> SHMNSEILNNIILNLRYRDNNLIDLSGYGANVEVYDGVELNDKNQFKLTSSTNSEIRVTQNQNIIFNSMFLDFSVSFWIRIPKYKNDGIQNYIHNEYTIINCIKNNSGWKISIRGNRIIWTLTDINGKTKSVFFEYSIREDISD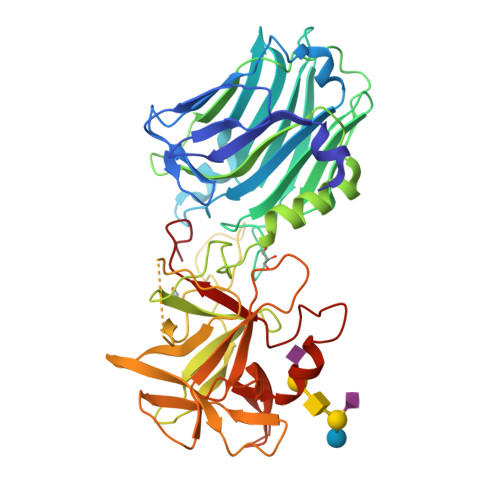YINRWFFVTITNNSDNAKIYINGKLESNIDIKDIGEVIANGEIIFKLDGDIDRTQFIWMKYFSIFNTELSQSNIKEIYKIQSYSEYLKDFWGNPLMYNKEYYMFNAGNKNSYIKLKKDSSVGEILTRSKYNQNSNYINYRNLYIGEKFIIRRKSNSQSINDDIVRKEDYIYLDFFNSNREWRVYAYKDFKEEEKKLFLANIYDSNEFYKTIQIKEYDEQPTYSCQLLFKKDEESTDEIGLIGIHRFYESGIVLKDYKNYFCISKWYLKEVKRKPYNPNLGCNWQFIPKDEGWIE4-(3,5-difluoro-4-hydroxybenzyl)-1,2-dimethyl-1H-imidazol-5-ol | C12 H12 F2 N2 O2 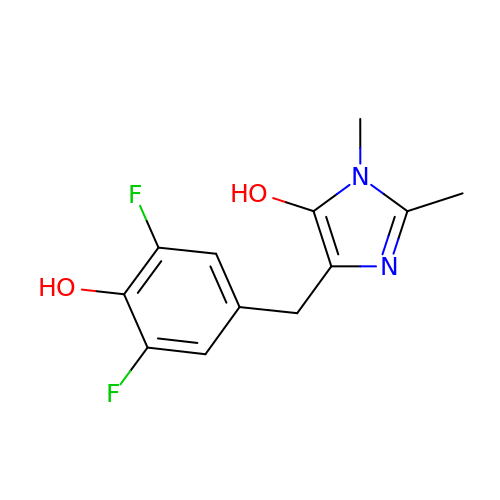| MSZRPLCUVKFQJC-UHFFFAOYSA-N> DMPVERILEAELAVEPKTETYVEANMGLNPSSPNDPVTNICQAADKQLFTLVEWAKRIPHFSELPLDDQVILLRAGWNELLIASFS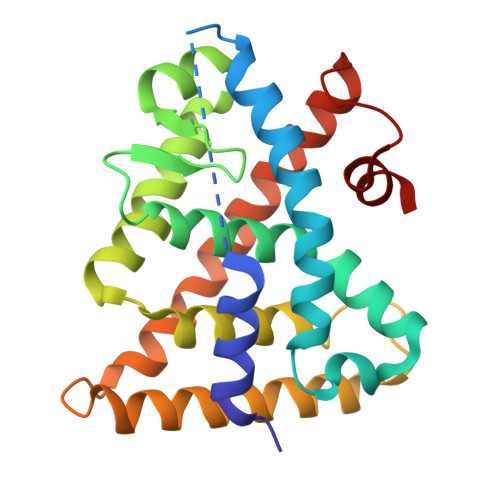HRSIAVKDGILLATGLHVHRNSAHSAGVGAIFDRVLTELVSKMRDMQMDKTELGCLRAIVLFNPDSKGLSNPAEVEALREKVYASLEAYCKHKYPEQPGRFAKLLLRLPALRSIGLKCLEHLFFFKLIGDTPIDTFLMEMLEA> LPLNSDYSLLLTFIYGGRVVGKTQVHSLDCRLVAERSDSESSMEQVEFPKPDPLEPTQHLLNQLDRGVLVASNSRGLFVQRLCPIPISWNAPEAPPGPGPHLLPSNKCVELFKTTYFCRDLAQYFQGQGPPPKFQATLHFWAASPGSSHSQENLITVQMEQAFARHLLEKI;> QLEIENRIQGLHVDIEFLVRSIRQLKDEQDVFSFRYTVFSLKKTSSSDPHQSQQAQLVQATANKVDRMRKEVLDISKGLVGRL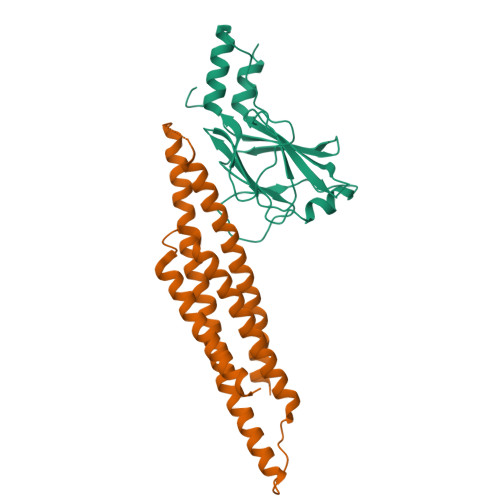TTLVDLLLPKLDEWKVQQAASCIGAPPPELQLEQLEQWLTAGAKFLFHLRQLLKQLKEMSHMLRYKGDMFGQGVDLQNAQVMELLQRLLQRS> TGRPEWIWLALGTALMGLGTLYFLVKGMGVSDPDAKKFYAITTLVPAIAFTMYLSMLLGYGLTMVPFGGEQNPIYWARYADWLFTTPLLLLDLALLVDADQGTILALVGADGIMIGTGLVGALTKVYSYRFVWWAISTAAMLYILYVLFFGFTSKAESMRPEVASTFKVLRNVTVVLWSAYPVVWLIGSEGAGIVPLNIETLLFMVLDVSAKVGFGLILLRSRAIFG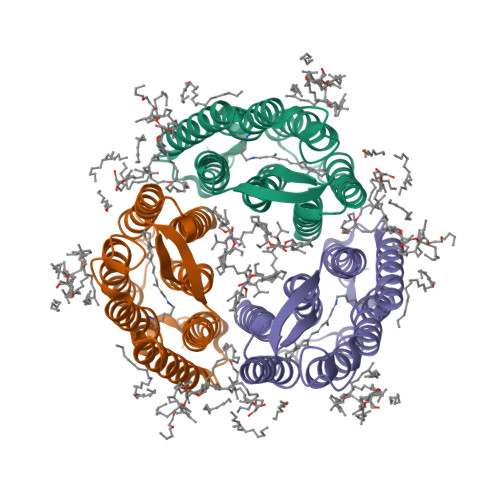EAE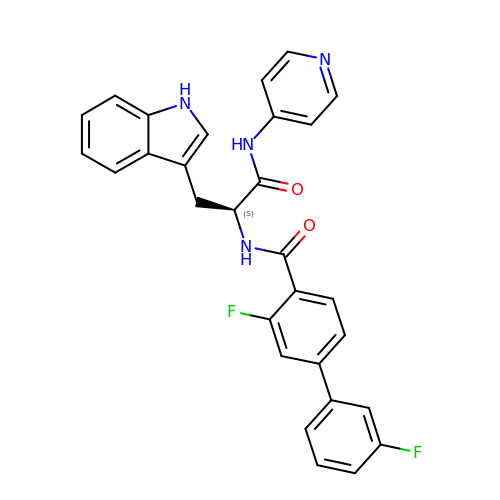3,3'-difluoro-N-[(2S)-3-(1H-indol-3-yl)-1-oxo-1-(pyridin-4-ylamino)propan-2-yl]biphenyl-4-carboxamide | C29 H22 F2 N4 O2 | QLYGOABRPGBQNG-MHZLTWQESA-N> MTTRPAESAPQTASTLLEPGSNGVVRLLGGPGTGKSSLLVDTAVQHILAGADPESVLLLTGSARLRTAARAAITARLLGAGTVGVVREPLVRTVHSYAFAVLRLAAQRNGDPPPRLITSAEQDGIIRELLAGDLEDGHRSPVGWPEQLWPALTTAGFATELRDLMARCTERGVDPIALQRLGRTAKRPEWLAAGRFAQAYEQIMLLRSAVGMAAPQATVPALGAAELVGAALEALGADDELLDTERNRIKLLLVDDAQHLDPQAARLVRALAAGTGLTVIAGDPDQSVFGYRGADPVLLRDDTHPAITLTQSYRCAPEIASAITGLGQRLPGVSDTRHWTGNPQREGTVTVRLAASTHAEGTMIADALRRAHLVDGIPWSQMAVIVRSVPRVGTALARALTAAGVPVQDNGTDVPVGRQPAAAALLTVLDVTATGHLDADSAVALLTGPIGRVDPVTLRQLRRALRRADGSQPPRDFGDLLVDAIEREPKGLSAEHARTLRRLRAVLTAARRSDASGADPRYTLWQAWHASGLQRRWLAASERGGSVGAQADRDLDAVTTLFDVADQYVNRTAGASLRGLVDHVTRLGAAVARTEPETAAEAVAVLSVHGALAGEWDFVVIAGVQEGLWPNMIPRGGVLGTQHLVDVLDGVADMTDRTVSTRAPLVAEERRLLMAAMGRARTRVMITAVDSDTGDESLLPSPFCAEISAWATEPVAEPPLVAPRVLAPSALVGRLRAVVCAPDGAVDDDARACAAAQLARLAAAGVPGADPSQWHAMTSLTTEEPLWSEPGHVVTLSPSTLQMLTDCPLRWLLERHGGDDGRDVRSTVGSLVHALVSEPGKTESQLVNELEKVWDDLPYDAKWYSDNELARHRAMLETFTRWREDTRRQLTEVATEIPVEGIVVEPGENTPGVRVRGRLDRLERDEAGRLVVVALKTGKSPVTKDDAQNHAQLAMYQLAVAAGLLDDGDEPGGGKLVYLGKAGAAGATEREQDPLTPDKRAEWLETVGEAAAATAGPRFVARVNNGCANCPVRSSCPAQANGDRP;> MTQVASPVVQARYSPVELSAALGLFPPTDEQAAVIAAPPGPLVVIAGAGAGKTETMAARVVWLVANGFATPSQVLGLTFTRKAAGQLLRRVRTRLARLAGAGLAPGSGASDESATVSTYHAFAGTLLREHGLLLPVEPDTRLLSETELWQLAYDVVCAHPGHLDTEKTPAAVTAMVLRLSGALAEHLVDTDQLRXXXXXXXXXXXXXXXXXXXXXXXXXXXLLRMLATQTERTELVPLIDALHQRMRAEKVMDF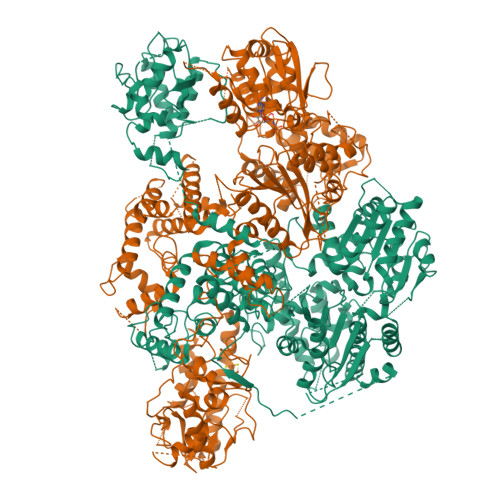GMQMAAAARLAARFPQVGEQLRQRFRVVLLDEYQDTGHAQRIALSSLFGGGADDGLALTAVGDPIQSIYGWRGASATNLPRFTTDFPYSDGTPAPTLELRTXXXXXXXXXXXXXXXXXXXXXXXXXXXXXXXXXXXXXXTIRCALLNNVAAERDWVADHLARAYHGAIGRGEAAPTAAVLVRRNADAAPMAEALTARGVPVEVVGVAGLLAVPEVADLVAMLRLIADPTAGSAVMRILTGPRWRFGARDIAALWRRAVELDDRPKGELGTADIVAQAAPDADTACVADAICDPGDAERYSPAGYERIVALGRELTMLRAHLGHPLPELVAEVRRVLGLDAEARAARPVAAGWAGTENLDRFSDLVSDFAGHAGASVSALLAYLDAAVEVENGLAPAELTVSHDRVQILTVHAAKGLEWQVVAVPHLSARVFPSTTQARTWLTDASDLPPLLRGDRATESEIGVPVLDTSDIYDRKILSDKISDHKKSLDQRRVDEERRLLYVAITRAEDTLLLSGHHWGATESKPRGPSEFLCELKTILEEATAAGTPCGEIEHWAPDPAPGETNPLRDQVVEALWPPVASADDHVHRGAQLVAAAMAGEVSAEADQEGWAADVDALLAERERPXXXXXXXXXXXXXXXXXXXXXXXXXXXXXXXXXXXXXXXXXHALLGTTFHEWVQRYFHAERLFDLDDLPGAVDSDSGRAVEESLAELQDAFVKSPWAARTPVEVEVPFDMVLGETVVRGRIDAVFAEPDGTTMVLAWKTGDPPETPEAKEHAAVQLAVYRLAWAAMRGCPPESVRAAFHYVRSGXXXXXXXXXXXXXXXXXLAAAPTETAEEADRIT>[2x]GSGEEVSEEGFQIPATITERYKVGRTIGDGNFAVVKECVERSTAREYALKIIKKSKCRGKEHMIQNEVSILRRVKHP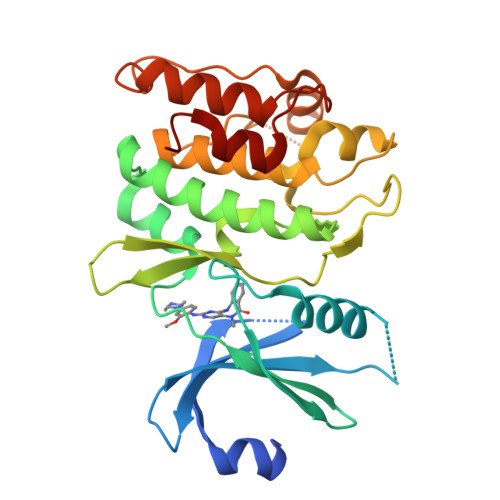NIVLLIEEMDVPTELYLVMELVKGGDLFDAITSTNKYTERDASGMLYNLASAIKYLHSLNIVHRDIKPENLLVYEHQDGSKSLKLGDFGLATIVDGPLYTVCGTPTYVAPEIIAETGYGLKVDIWAAGVITYILLCGFPPFRGSGDDQEVLFDQILMGQVDFPSPYWDNVSDSAKELITMMLLVDVDQRFSAVQVLEHPWVND>MGHHHHHHMGFEGLADRLQQTISKIRGKGKVSEQDVKEMMREVRLALLEADVNFKVVKDFVKKVSERAVGQDVMKSLTPGQQVIKVVQEELTELMGGEESKIAVAKRPPTVIMMVGLQGAGKTTTSGKLANLLRKKHNRKPMLVAADIYRPAAIKQLETLGKQLDMPVFSLGDQVSPVEIAKQAIEKAKEEHYDYVILDTAGRLHIDHELMDELTNVKEIANPEEIFLVVDSMTGQDAVNVAKSFNEQLGLTGVVLTKLDGDTRGGAALSIRAVTNTPIKFAGLGEKLDALEPFHPERMASRILGMGDL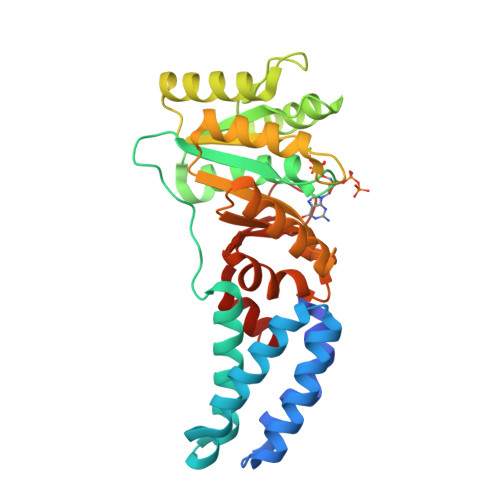E[3x]> GHMKQEELKRLYKAQAIQRQLEEVEERQRASEIQGVRLEKALRGEADSGTQDEAQLLQEWFKLVLEKNKLMRYESELLIMAQELELEDHQSRLEQKLREKMLKEESQKDEKDLNEEQEV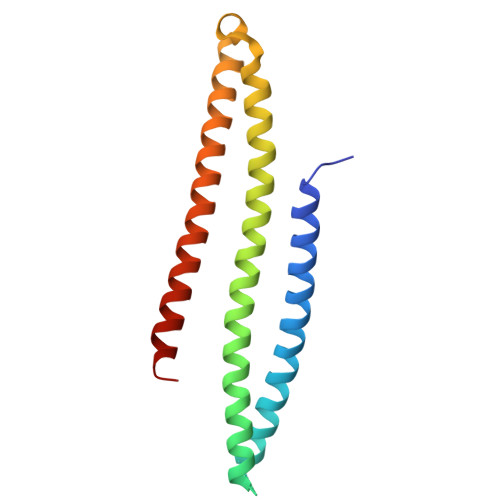FTELMQVIEQRDKLVDSLEEQRIREKAEDQHFES> GSKDYDELLKYYELHETIGTGGFAKVKLACHILTGEMVAIKIMDKNTLGSDLPRIKTEIEALKNLRHQHICQLYHVLETANKIFMVLEYCPGGELFDYIISQDRLSEEETRVVFRQIVSAVAYVHSQGYAHRDLKPENLLFDEYHKLKLIDFGLCAKPKGNKDYHLQTCCGSLAYAAPELIQGKSYLGSEADVWSMGILLYVLMCGFLPFDDDNVMALYKKIMRGKYDVPKWLSPSSILLLQQMLQVDPKKRISMKNLLNHPWIMQDYNYPVEWQSKNPFIHLDDDCVTELSVHHRNNRQTMEDLISLWQYDHLTATYLLLLAKKARGKPVRLRLSSFSCG

Maternal embryonic leucine zipper kinase (MELK) is a serine/threonine kinase in the adenosine monophosphate-activated protein kinase (AMPK)-related kinase family, and was first identified as a maternal gene in mouse eggs and preimplantation embryos. Out of all of these potential roles, MELK is best characterized as a mitotic kinase, as its expression pattern highly correlates with other mitotic genes. At the protein level, MELK is hyperphosphorylated, and reaches its maximal abundance and kinase activity during M phase in both Xenopus embryos and human cancer cell lines. Due to the potential oncogenic role of MELK, several groups have developed MELK inhibitors to validate its potential as a drug target.

Here, we report the discovery of HTH-01-091, a potent and selective MELK inhibitor. HTH-01-091 inhibits MELK with an IC50 value of 10.5 nM, which is comparable to MELK-T1 and NVS-MELK8a in the same enzymatic assay. To better understand the mode of inhibitor binding, we determined crystal structures of MELK in complex with HTH-01-091 and MRT199665. The 2.5 Å structure of MELK in complex with HTH-01-091 revealed a type I binding mode. The quinoline nitrogen in the tricylic core forms the only hinge interaction with the backbone NH of Cys89. In the deep pocket, the 3,5-dichloro-4-hydroxyphenyl group engages with the catalytic (Lys40) lysine and recruits Glu57 on the αC helix. Toward the solvent, the cyclic urea group forms a hydrogen bond with Ile17 in the P-loop. In addition, the cyclohexyl group of HTH-01-091 is sandwiched between Val25 and Leu139 in a nearly orthogonal orientation with respect to the core, while projecting the (dimethylamino)methyl tail into the negatively-charged catalytic pocket made-up by Glu93, Asp150, and Glu136. Many of the corresponding interactions were previously observed in the MELK-OTSSP167 co-crystal structure. However, in the OTSSP167 structure, the cyclohexyl group occupies the active site in a manner that makes greater van der Waals interactions with the P-loop, causing the N-lobe to be in a slightly more closed conformation reflected by the proximity of Phe22 to the carboxyl end of the αC helix.>[4x]MARPKSEDKKQALLEAATQAIAQSGIAASTAVIARNAGVAEGTLFRYFATKDELINTLYLHLTQDWCQSIIMELDRSITDAKMMTRFLWNSWISWGLNHPARHRAIRQLAVSE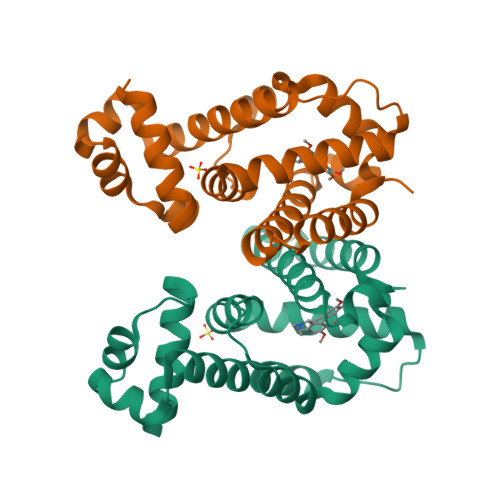KLTKETEQRADDMFPELRDHLHRNVLMVFMSDEYRAFGDGLFLALAETTMDFAARDPARAGEYIALGFEAMWRALAREEQ> MAKRRNRKTRFNLPPGKSGWPFLGETIGYLKPYTATTLGDFMQQHVSKYGKIYRSNLFGEPTIVSADAGLNRFILQNEGRLFECSYPRSIGGILGKWSMLVLVGDMHRDMRSISLNFLSHARLRTILLKDVERHTLFVLDSWQQNSIFSAQDEAKKFTFNLMAKHIMSMD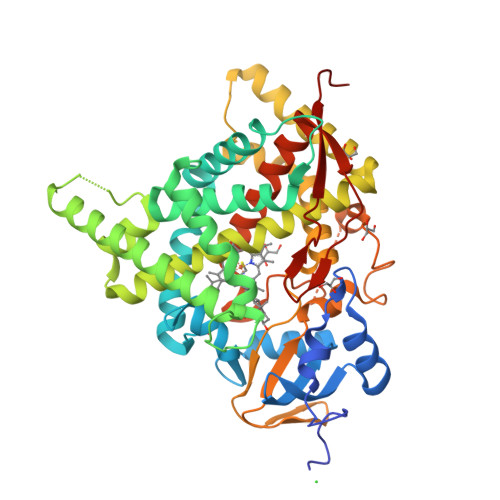PGEEETEQLKKEYVTFMKGVVSAPLNLPGTAYHKALQSRATILKFIERKMEERKLDIKERKQRTDDDLLGWVLKHSNLSTEQILDLILSLLFAGHETSSVAIALAIFFLQACPKAVEELREEHLEIARAKKELGESELNWDDYKKMDFTQCVINETLRLGNVVRFLHRKALKDVRYKGYDIPSGWKVLPVISAVHLDNSRYDQPNLFNPWRWQQQTWGNNYMPFGGGPRLCAGSELAKLEMAVFIHHLVLKFNWELAEDDKPFAFPFVDFPNGLLIRVSRILHHHH5-(FORMYLAMINO)-1-(5-O-PHOSPHONO-BETA-D-RIBOFURANOSYL)-1H-IMIDAZOLE-4-CARBOXYLIC ACID | C10 H14 N3 O10 P | 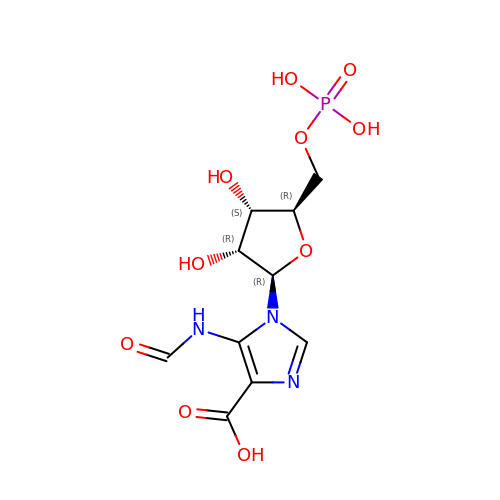UEBVPQPUWAADHX-FJGDRVTGSA-N>[2x]MAHERMTPATACIHANPQKDQFGAAIPPIYQTSTFVFDN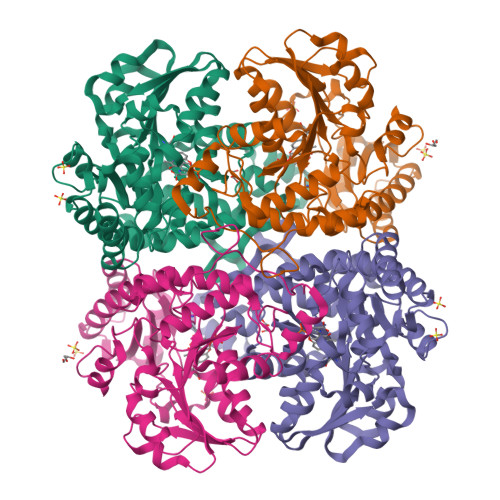CQQGGNRFAGQESGYIYTRLGNPTVSNLEGKIAFLEKTEACVATSSGMGAIAATVLTILKAGDHLISDECLYGCTHALFEHALTKFGIQVDFINTAIPGEVKKHMKPNTKIVYFETPANPTLKIIDMERVCKDAHSQEGVLVIADNTFCSPMITNPVDFGVDVVVHSATKYINGHTDVVAGLICGKADLLQQIRMVGIKDITGSVISPHDAWLITRGLSTLNIRMKAESENAMKVAEYLKSHPAVEKVYYPGFEDHEGHDIAKKQMRMYGSMITFILKSGFEGAKKLLDNLKLITLAVSLGGCESLIQHPASMTHAVVPKEEREAAGITDGMIRLSVGIEDADELIADFKQGLDALLRSHHHHHH>[2x]MISLQSDQLLEATVGQFMIEADKVAHVQVGNNLEHALLVLTKTGYTAIPVLDPSYRLHGLIGTNMIMNSIFGLERIEFEKLDQITVEEVMLTDIPRLHINDPIMK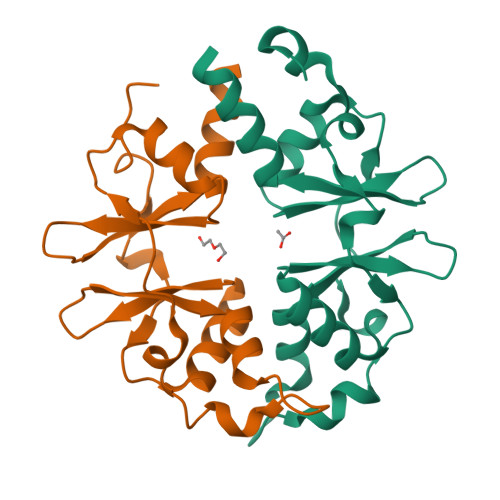GFGMVINNGFVCVENDEQVFEGIFTRRVVLKELNKHIRSLNK>[2x]LSTCTTLDFGHIKKKRVEAIRGQILSKLRLTSPPEPTVMTHVPYQVLALYNSTRELLEEMHGEREEGCTQENTESEYYAKEIHKFDMIQGLAEHNELAVCPKGITSKVFRFNVSSVEKNRTNLFRAEFRVLRVPNPSSKRNEQRIELFQILRPDEHIAKQRYIGGKNLPTRGTAEWLSFDVTDTVREWLLRRESNLGLEISIHCPCHTFQPNGDILENIHEVMEIKFKGVDNEDDHGRGDLGRLKKQKDHHNPHLILMMIPPHRLDNPGQGGQRKKRALDTNYCFRNLEENCCVRPLYIDFRQDLGWKWVHEPKGYYANFCSGPCPYLRSADTTHSTVLGLYNTLNPEASASPCCVPQDLEPLTILYYVGRTPKVEQLSNMVVKSCKCS;> HQDKVPCKMVDKKVSCQVLGLLQVPSVLPPDTETLDLSGNQLRSILASPLGFYTALRHLDLSTNEISFLQPGAFQALTHLEHLSLAHNRLAMATALSAGGLGPLPRVTSLDLSGNSLYSGLLERLLGEAPSLHTLSLAENSLTRLTRHTFRDMPALEQLDLHSNVLMDIEDGAFEGLPRLTHLNLSRNSLTCISDFSLQQLRVLDLSCNSIEAFQTASQPQAEFQLTWLDLRENKLLHFPDLAALPRLIYLNLSNNLIRLPTGPPQDSKGIHAPSEGWSALPLSAPSGNASGRPLSQLLNLDLSYNEIELIPDSFLEHLTSLCFLNLSRNCLRTFEARRLGSLPCLMLLDLSHNALETLELGARALGSLRTLLLQGNALRDLPPYTFANLASLQRLNLQGNRVSPCGGPDEPGPSGCVAFSGITSLRSLSLVDNEIELLRAGAFLHTPLTELDLSSNPGLEVATGALGGLEASLEVLALQGNGLMVLQVDLPCFICLKRLNLAENRLSHLPAWTQAVSLEVLDLRNNSFSLLPGSAMGGLETSLRRLYLQGNPLSCCGNGWLAAQLHQGRVDVDATQDLICRFSSQEEVSLSHVRPEDCEKGGLKNIN

Transforming growth factor-β (TGF-β1) is a multifunctional cytokine with key roles in development, immunity, cancer, and fibrosis. Latency of mature TGF-β is determined by non-covalent association with its N-terminal prodomain cleaved by furin during biosynthesis. The prodomain encircles mature TGF-β homodimer in a ring-shaped disulfide linked homodimer “straitjacket”, (latency-associated peptide, LAP), forming L-TGF-β5. Interestingly, both TGF-β1 and -β3 LAPs contain the integrin binding motif RGDLXXL/I and bind to two integrins, αvβ6 and αvβ8, which together account for the majority of TGF-β1, and some of TGF-β3 function, in vivo.

Single particle cryo-EM studies provided structures of L-TGF-β3/GARP (2.9Å), comparable with that of L-TGF-β1/GARP (3.0Å). The portion of the straitjacket in contact with GARP almost identical in both structures. However, L-TGF-β3 is significantly more flexible in all other regions by B-factor comparison to L-TGF-β1, particularly the arm, which contains the integrin binding site, and the portion of the straitjacket domain, including the lasso loop, that cradles the tip of mature TGF-β containing the receptor binding domain. Such increased intrinsic flexibility suggests that L-TGF-β3 is less constrained and contains higher basal entropy than L-TGF-β1. We hypothesize that increased basal entropy facilitates exposing mature TGF-β3 to TGF-βRs even without binding to αvβ8. To test this, we expressed L-TGF-β3/GARP and measured TGF-β activation using TMLC reporter cells, which, indeed, has significantly higher detectable basal TGF-β activity than that of L-TGF-β1/GARP with no basal activity. A detailed comparison of sequence and structure reveals that the lasso loop of L-TGF-β3 (lasso) is not only shorter than L-TGF-β1 (lasso) but also less conserved in key residues interacting with mature TGF-β53. The high basal activity of L-TGF-β3 was unexpected, which we attribute to the increased intrinsic entropy of straitjacket and lasso loops compared to TGF-β1.> MDEKLLKTIAESKYLVALTGAGVSAESGIPTFRGKD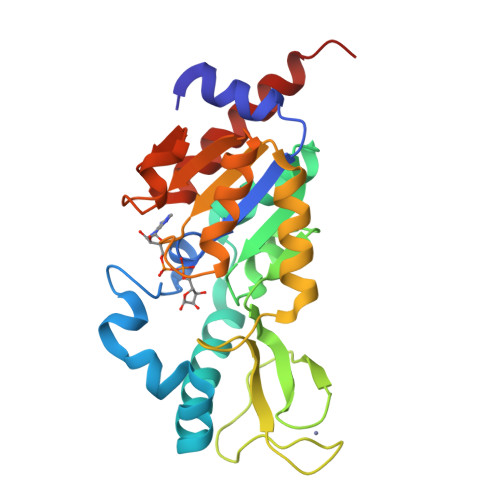GLWNRYRPEELANPQAFAKDPEKVWKWYAWRMEKVFNAQPNKAHQAFAELERLGVLKCLITQNVDDLHERAGSRNVIHLHGSLRVVRCTSCNNSFEVESAPKIPPLPKCDKCGSLLRPGVVWAGEMLPPDVLDRAMREVERADVIIVAGTSAVVQPAASLPLIVKQRGGAIIEINPDETPLTPIADYSLRGKAGEVMDELVRHVRKALSLKLN>GSMKLFAQGTSLDLSHPHVMGILNVTPDSFSDGGTHNSLIDAVKHANLMINAGATIIDVGGESTRPGAAEVSVEEELQRVIPVVEAIAQRFEVWISVDTSKPEVIRESAKVGAHIINDIRSLSEPGALEAAAETGLPVCLMHMQGNPKTMQEAPKYDDVFAEVNRYFIEQIARCEQAGIAK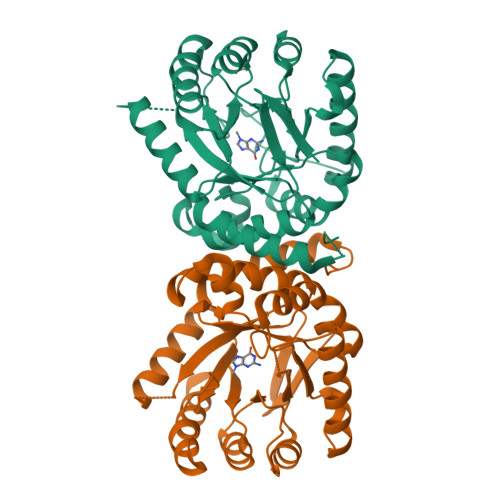EKLLLDPGFGFGKNLSHNYSLLARLAEFHHFNLPLLVGMSRKSMIGQLLNVGPSERLSGSLACAVIAAMQGAHIIRVHDVKETVEAMRVVEATLSAKENKRYE[2x]> TNEY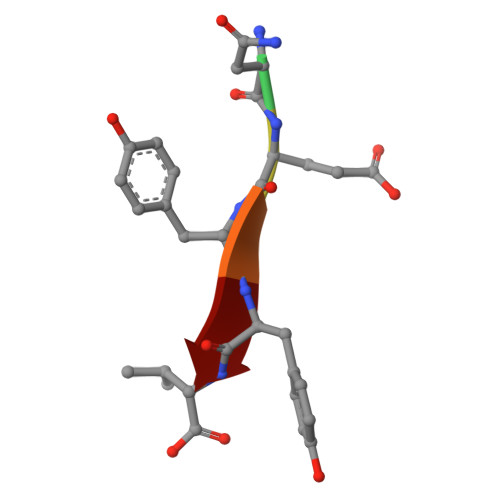YV> MYYGISQFSEAYNKILRNSSSHSSCQLVIFVSCLNIDALCATKMLSLLFKKQLVQSQIVPIFGYSELRRHYSQLDDNINSLLLVGFGGVIDLEAFLEIDPQEYVIDTDEKSGEQSFRRDIYVLDAHRPWNLDNIFGSQIIQCFDDGTVDDTLGEQKEAYYKLLELDEESGDDELSGDENDNNGGDDEATDADEVTDEDEEDEDETISNKRGNSSIGPNDLSKRKQRKKQIHEYEGVLEEYYSQGTTVVNSISAQIYSLLSAIGETNLSNLWLNILGTTSLDIAYAQVYNRLYPLLQDEVKRLTPSSRNSVKTPDTLTLNIQPDYYLFLLRHSSLYDSFYYSNYVNAKLSLWNENGKKRLHKMFARMGIPLSTAQETWLYMDHSIKRELGIIFDKNLDRYGLQDIIRDGFVRTLGYRGSISASEFVEALTALLEVGNSTDKDSVKINNDNNDDTDGEEEEDNSAQKLTNLRK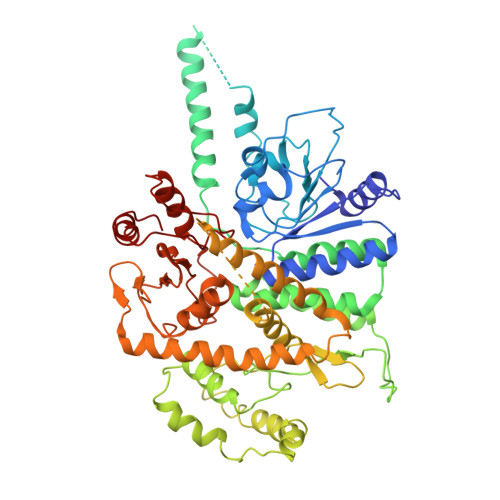RWVSNFWLSWDALDDRKVELLNRGIQLAQDLQRAIFNTGVAILEKKLIKHLRIYRLCVLQDGPDLDLYRNPLTLLRLGNWLIECCAESEDKQLLPMVLASIDENTDTYLVAGLTPRYPRGLDTIHTKKPILNNFSMAFQQITAETDAKVRIDNFESSIIEIRREDLSPFLEKLTLSGLL In this work, we exhaustively probe the ability of all 36 immobile HJ sequences to form DNA crystals in two different designed systems. Three separate self-assembling DNA crystal systems are described in this report: the “4 × 5” and “4 × 6” designs (collectively referred to as the 4 × N systems), and a third construct with a “scrambled” sequence variant of the 4 × 6 lattices. Self-assembly was mediated by three constituent oligonucleotides: (S1) containing four sequence repeats of either 5 or 6 bases; (S2) composed of 21 bases containing complementary regions to both (S1); and (S3) which forms the second junction crossover. The HJ serves as the fundamental component at the core of each unit, and the ultimate assembly of the full lattice is facilitated by the complementary 2-base sticky ends that tail each duplex.

Each asymmetric unit could be defined as either a HJ containing 10 and 11 bp on each arm, or as a 21-bp linear duplex. In parallel, we employed the previously reported J1 4 × 6 system (3.05 Å), with P32 symmetry. Seventeen of the 36 junctions successfully crystallized, a 47% success rate. Unlike the 4 × 5 motif, nearly all of the 4 × 6 junction sequences had a strong preference for crystallization in buffers containing ≥2.0 M salts (e.g., LiCl, Li2SO4, KCl, and NaCl), with the majority preferring slightly basic pH conditions in cacodylic acid. The average cell constants for the P32 crystals were a = b = 68.29 Å c = 55.68 Å. The c-axis, in particular, was ~5 Å shorter, and had a much larger degree of variability (σ = 1.97), than those that crystallized using the 4 × 5 motif. The broad range of the short axis spanned from 52.77 to 60.36 Å, and we posit that the flexible axis lengths could be responsible for rendering a larger number of junctions fatal than the 4 × 5 system. The average junction angles of 54.60° (σ = 1.44) and 58.37° (σ = 2.3) for the P32 and R3 symmetries, respectively, along with their preference for salts or organic solvents, were likely the major contributing factors that yielded the divergent lattices. However, in the majority of the crystal structures reported here, the cacodylate anion indeed fits best into the electron density map of our X-ray structures, due to the presence of sodium cacodylate in the crystallization solution.

> GAGCAGACTTGACGACACTCA;> TCGTCA;> TCTGAGTG;> AGTCTGC>MAHHHHHHVDDDDKMVPPKKDMEKGVIFSDLCNFLITQTLQGWKVYWAGIEFDVSQKGMALLTRLKTNDFAPAWAMTRNLFPHLFQNPNSVIQSPIWALRVILAAGLQDQLLDHSLVEPLTGALGLISDWLLTTTSTHFNLRTRSVKDQLSLRMLSLIRSN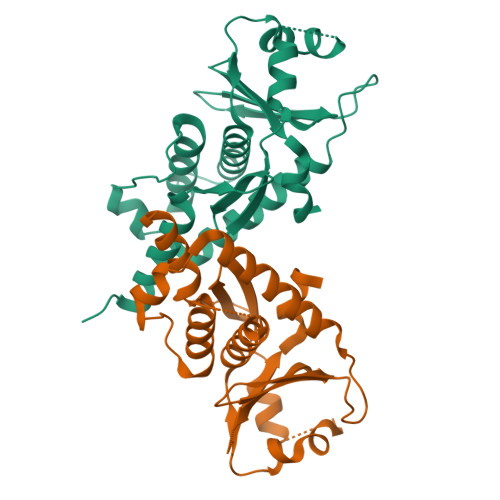ILQFINKLDALHVVNYNGLLSSIEIGTSTHTIIITRTNMGFLVEVQEPDKSAMNSKRPGPVKFSLLHESAFKPFT[2x]> MNTPEHMTAVVQRYVAALNAGDLDGIVALFADDATVEDPVGSEPRSGTAAIREFYANSLKLPLAVELTQEVRAVANEAAFAFTVSFEYQ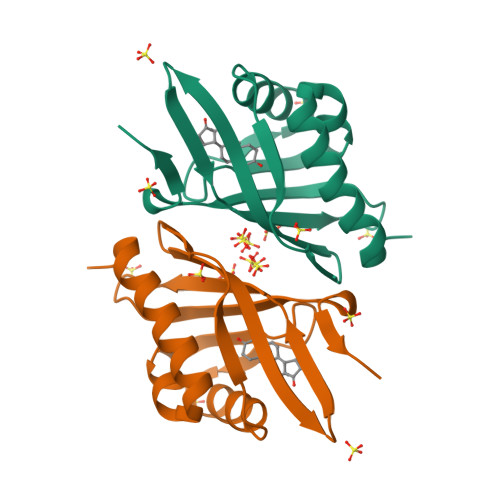GRKTVVAPINHFRFNGAGKVVSMRALFGEKNIHAGA> GSPALDTGTTEEDRLKIDVIDWLVFDPAQRAEALKQGNAIMRKFLASKKHEAAKEVFVKIPQDSIAEIYNQCEEQGMESPLPAEDDNAIREHLCIRAYLEAHETFNEWFKHMNSVPQKPALIPQPTFTEKVAHEHKEKKYEMDFGIWKGHLDALTADVKEKMYNVLLFVDGGWMVDVREDAKEDHERTHQMVLLRKLCLPMLCFLLHTILHSTGQYQECLQLADMVSSERHKLYLVFSKEELRKLLQKLRESSLMLLDQGLDPLGYEIQL;> MASHMLSWLHEINSQELEKAHATLLGLANMETRYFAKKKTLLGLSKLAALASDFSEDMLQEKIEEMAEQERF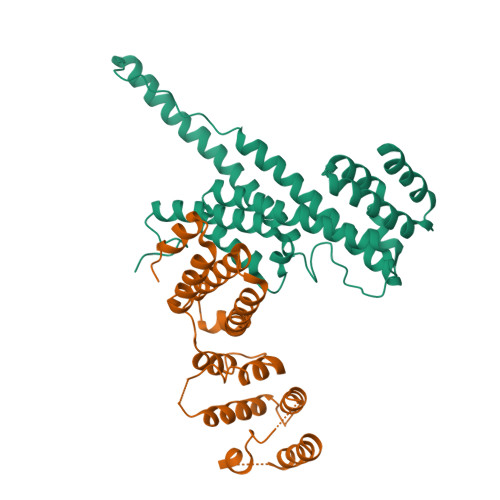LLHQETLPEQLLAEKQLNLSAMPVLTAPQLIGLYICEENRRANEYDFKKALDLLEYIDEEEDININDLKLEILCKALQRDNWSSSDGKDDPIEVSKDSIFVKILQKLLKDGIQLSEYLPEVKDLLQADQLGSLKSNPYFEFVLKANYEYYVQGQI> MKVAVLPGDGIGPEVTEAALKVLRALDEAEGLGLAYEVF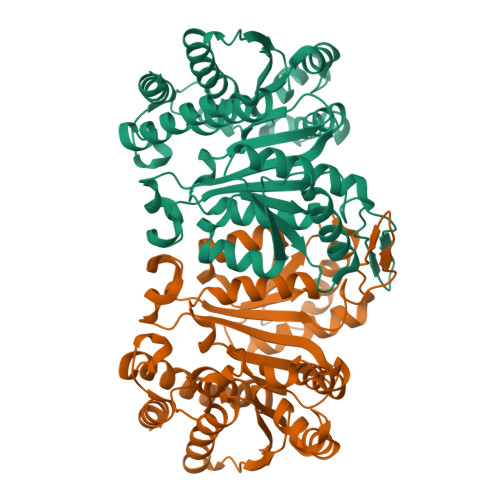PFGGAAIDAFGEPFPEPTRKGVEEAEAVLLGSVGGPKWDGLPRKIRPETGLLSLRKSQDLFANLRPAKVFPGLERLSPLKEEIARGVDVLIVRELTGGIYFGEPRGMSEAEAWNTERYSKPEVERVARVAFEVARKRRKHVVSVDKANVLEVGEFWRKTVEEVGRGYPDVALEHQYVDAMAMHLVRSPARFDVVVTGNIFGDILSDLASVLPGSLGLLPSASLGRGTPVFEPVHGSAPDIAGKGIANPTAAILSAAMMLEHAFGLVELARKVEDAVAKALLETPPPDLGGSAGTEAFTATVLRHLA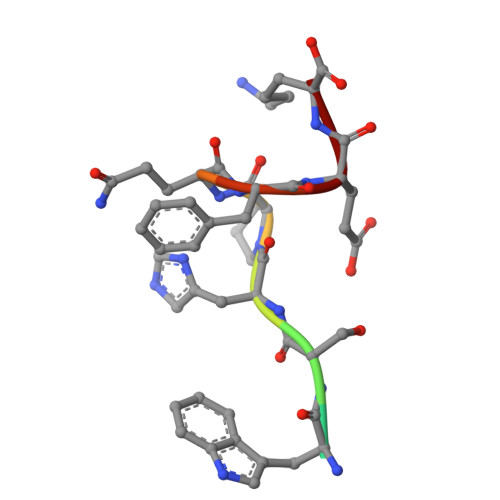> SNWSHPQFEK(2R)-2,3-DIHYDROXYPROPANOIC 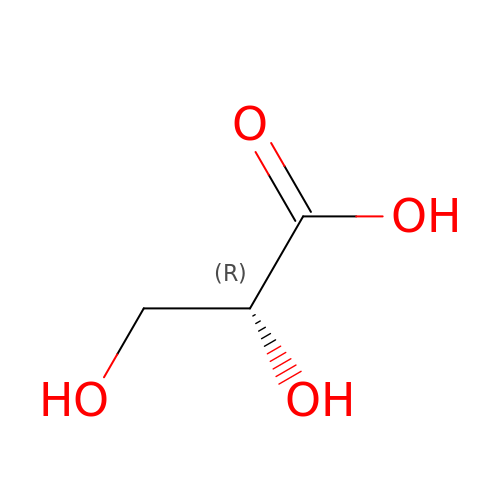ACID | C3 H6 O4 | RBNPOMFGQQGHHO-UWTATZPHSA-N> ARLAGKVAIVTGGVNGIGLAIANKFVEEGANVVITGSHALVGQKAAASIGGVNVIRFVEHNASDEAGWVALFNVTSAAFGPVVTVVDNAGIAVSKSTEDVTTAEWKSLLVVNLLGVFFGTRNGIERMKNKGLGASIINMSTIEGFTGN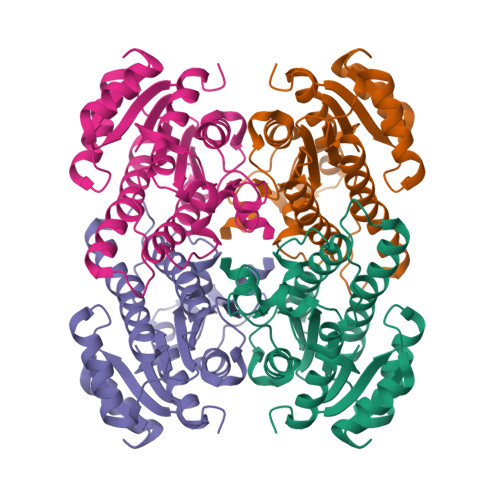PVLGAYLASKGAVRIQSKSAALDSADKNYNVRVDTVHPGYIKTPLVDKAAGAEESMSQRTSVPMGHIGTPLDIAWISVYDATDESKFAVGAKFVVDGGYVAE> GMIKKISVVLVLLTGMLLSASVFAQKTIVEKYGKLSVKGNYMVGQYGDTVQLRGMSLFWSQWMGQYYNSDVVKWLRDDWKCTVVRAAMGVEMDGYLENPDTEKMKVMEVVNAAIAKGIYVIIDYHSHEAQKNPAAAQRF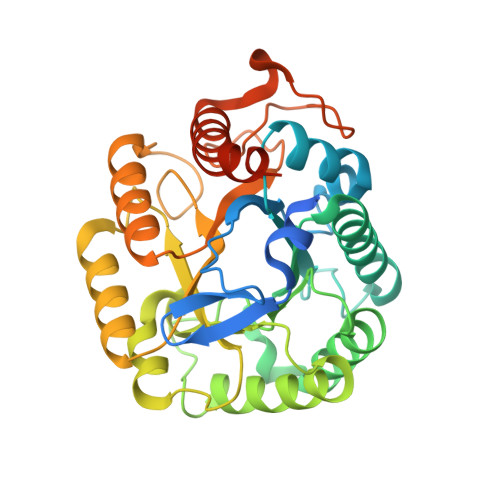FSEMAKKYGNIPNIIYEVYNEPLQATSWNKDIKPYAEGVITKIRVYDTTNIIVVGTRQWSQLVTEAAANPITRQNIMYTLHFYPGTHKQELRNEAQKALDMGIALFVTEYGTCDASGNGNFSPEETALWYEFLDAHKISYCNWSIADKPETASAIVPAASPYGGWADYDLTPSGKLVRDDLRLKNGPIFDSLVKTSTGGVSKKKSKTK>MWRKLMGERGEVYSEKLFTESERTYFFNVKENRKGDYFLNIVESKRSPSGDFERHSIFVYEENINEFESNLLKAIAVIKQKVSTGSVGSSARHNKGYGEYGERSKLDDSRFDKKSHLSGGRFKKKDY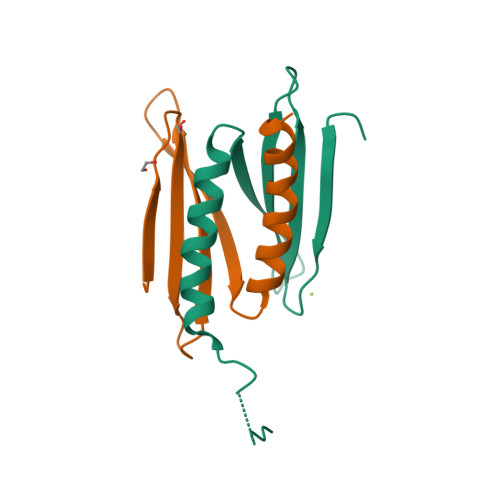[4x]> IATPNKSKSTKPTSENPKIGPI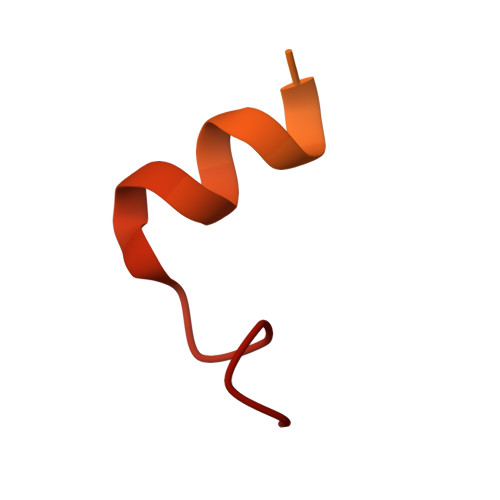SEVASGVKTAANGIERIPVLGEIAKPVTAAVKWFADIVGGVAAIFGW(2~{S})-2-azanyl-4-sulfo-butanoic 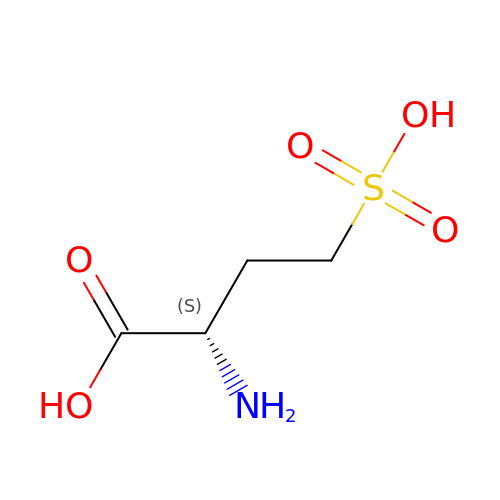acid | C4 H9 N O5 S | VBOQYPQEPHKASR-VKHMYHEASA-N>[4x]GPAAPAQSPAAPDPEASPLAEPPQEQSLAPWSPQTPAPPCSRCFARAIESSRDLLHRIKDEVGAPGIVVGVSVDGKEVWSEGLGYADVENRVPCKPETVMRIASISKSLTMVALAKLWEAGKLDLDIPVQHYVPEFPEKEYEGEKVSVTTRLLISHLSGIRHYEKDIKKVKEEKAYKALKMMKENVAFEQEKEGKSNEKNDFTKFKTEQENEAKCRNSKPGKKKNDFEQGELYLREKFENSIESLRLFK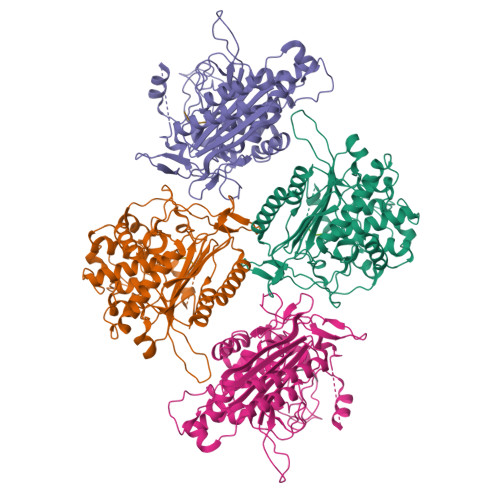NDPLFFKPGSQFLYSTFGYTLLAAIVERASGCKYLDYMQKIFHDLDMLTTVQEENEPVIYNRARFYVYNKKKRLVNTPYVDNSYKWAGGGFLSTVGDLLKFGNAMLYGYQVGLFKNSNENLLPGYLKPETMVMMWTPVPNTEMSWDKEGKYAMAWGVVERKQTYGSCRKQRHYASHTGGAVGASSVLLVLPEELDTETINNKVPPRGIIVSIICNMQSVGLNSTALKIALEFDKDRSD;>[4x]AAS> MNTIAWLGRLVIERIRGIGVAALMLLQIIFSLPSAGGFGRFVYQMHRVGVMSLLIITVSGLFIGLVLGLQGYSILVNVGSESMLGTMVSLTLLRELAPVVAALLFAGRAGSALTAEIGSMKQSEQLASMEMIGVDPLKQIVSPRLWAGIVSLPMLTVIFAAIGIVGGKLVGVDFLGVDEGSFWSGMQNNVQFGHDV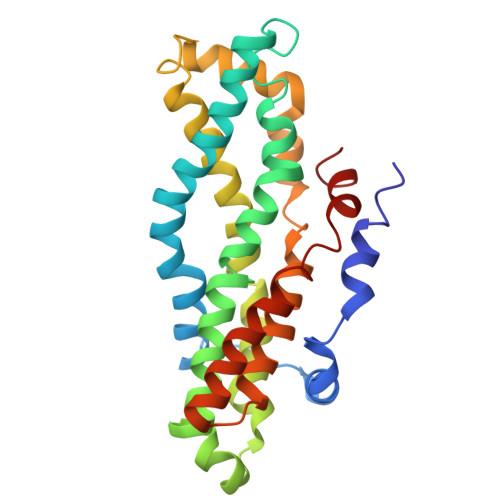VNGIIKSIVFALLCTWIAVFQGYACDPTPEGIATAMTRTVVYSSLCVLGFDFVLTAVMFGG> MELKNSISDYTEAEFVQLLKEIEKENVAATDDVLYVLL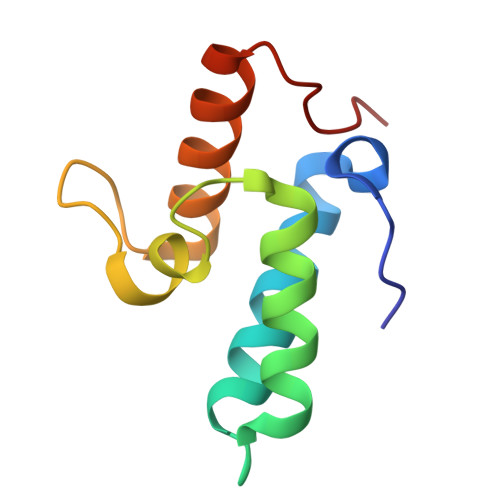EHFVKITEHPDGTDLIYYPSDNRDDSPEGIVKEIKEWRAANGKPGFKQG> MKCLVTGGNVKVLGKAVHSLS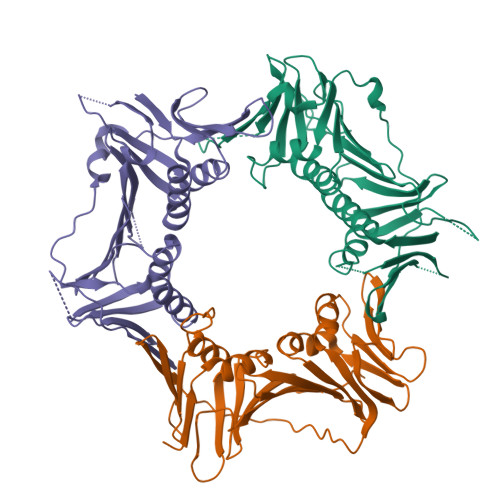RIGDELYLEPLEDGLSLRTVNSSRSAYACFLFAPLFFQQYQAATPGQDLLRCKILMKSFLSVFRSLAMLEKTVEKCCISLNGRSSRLVVQLHCKFGVRKTHNLSFQDCESLQAVFDPASCPHMLRAPARVLGEAVLPFSPALAEVTLGIGRGRRVILRSYHEEEADSTAKAMVTEMCLGEEDFQQLQAQEGVAITFCLKEFRGLLSFAESANLNLSIHFDAPGRPAIFTIKDSLLDGHFVLATLSDTDSGTTSTSLEVLFQGPLSGSGGHHHHHH;> MPLLTQQIQDEDDQYSLVASLDNVRNLSTILKAIHFREHATCFATKNGIKVTVENAKCVQANAFIQAGIFQEFKVQEESVTFRINLTVLLDCLSIFGSSPMPGTLTALRMCYQGYGYPLMLFLEEGGVVTVCKINTQEPEETLDFDFCSTNVINKIILQSEGLREAFSELDMTSEVLQITMSPDKPYFRLSTFGNAGSSHLDYPKDSDLMEAFHCNQTQVNRYKISLLKPSTKALVLSCKVSIRTDNRGFLSLQYMIRNEDGQICFVEYYCCPDEEVPESES;> MKFRAKIVDGACLNHFTRISNMIAKLAKTCTLRISPDKLNFILCDKLANGGVSMWCELEQENFFNEFQMEGVSAENNEIYLELTSENLSRALKTAQNARALKIKLTNKHFPCLTVSVELLSMSSSSRIVTHDIPIKVIPRKLWKDLQEPVVPDPDVSIYLPVLKTMKSVVEKMKNISNHLVIEANLDGELNLKIETELVCVTTHFKDLGNPPLASESTHEDRNVEHMAEVHIDIRKLLQFLAGQQVNPTKALCNIVNNKMVHFDLLHEDVSLQYFIPALS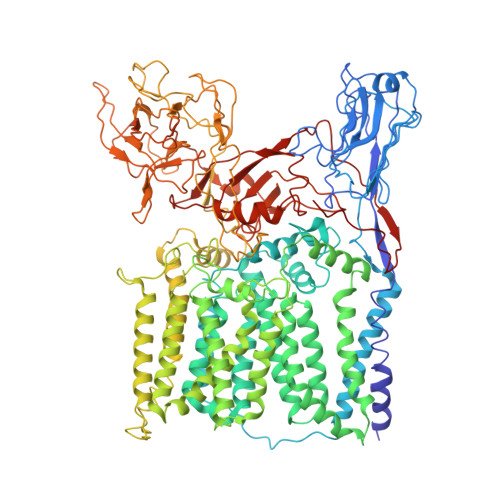> DYKDDDDKMTEPSRIARLIAVVAGIAGVLLCGLVPLLPVEETTATVLWPQGVGADGNVTELTAPLVAGAPRALDVTIPCRAVAELPADGGVVFSTNPAGGIEAGRNGMFIRANADVVYVAFRDTVAAVAPREAVDSGACSEIHVWADVSAVGADFAGIPDASGTLPVDKRPQVSGVFTDLKVPAQPGLAARIDIDTRFITSPTLLKTAVMVLGLACVIGSIVALALLDRGWRRRPPRTRGRAGLWTWITDTGVIGGLLIWHIVGAPTSDDGYNMTIARVASEAGYTTNYYRYFGASEAPFDWYQSVLSHLASISTAGVWMRLPATAAAIATWLIISRCVLPRIGRRVAANRVAMLTAGATFLAAWLPFNNGLRPEPLIAFAVITVWMLVENSIGTRRLWPAAVAIVIAMFSVTLAPQGLIALAPLLVGARAIGRVVTARRAGTGILASLAPLAASVAVVFVIIFRDQTLATVAESVRIKYVVGPTIPWYQEFLRYYFLTVEDSVDGSLTRRFAVLVLLLCLFGLIMVLLRRGRVPGAVSGPLWRLCGSTAIGLLLLILTPTKWAIQFGAFAGLAGALGGVTAFAFARVGLHSRRNLALYVTALLFILAWATSGLNGWFYVGNYGVPWFDKQPVIAHYPVTTIFLVLAIVGGLLAGWLHFRMDYAGHTEVADTGRNRALASTPLLIVATIMVVLELGSMVKATVGRYPVYTVGSANIAALRSAGDSCAMADAVLVEADPNEGMLQPVPGQRFGEYGPLGGEDPVGFTPNGVSDTLEPAEPVAANPGTPNSDGPVDKPNIGIGYAAGTGGGYGPEGVNGSRVFLPFGLDPSRTPVMGSYGENKLAAKATSAWYQLPPRTPDRPLVTVAAAGAIWYYEEDGSFNYGQSLKLQWGVHRPDGTYQALSEVQPIDIFQQKAWRNLRFPLAWAPPEANVARIVADDPNLSEDQWFAFTPPRVPVLQTAQQFLGSQTPVLMDIATAANFPCQRPFAERLGVAELPEYRIIPNFKQMVVSSNQWQSAADGGPFLFIQALLRTEAIPTYLRDDWYRDWGSIERYIRVVPQEQAPTAAIEEGSTRVFGWSRGGPIRALP>[4x]MAH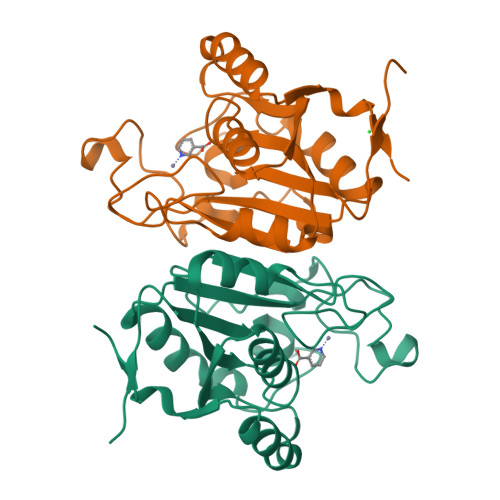HHHHHVGTGSNDDDDKSPDPPTLCVTVSSTTDVLIIADMQVDFLAPGGSLHVKGGEALLDGINAVSSQLPFRYQVATQDWHPENHCSFVTHGGPWPPHCVQGSAGAQLHAGLHTQRINAVIRKGVTQQADSYSAFVEDNGVSTGLAGLLHSIGARRVFVCGVAYDFCVFFTAMDARKNGFSVVLLEDLTAAVDDAAWSARTAELKDAGVVLLKSSALVAEGTQT>MGMEFSSHHIRLLQQLDEQRQKDLFCDCHIIVEGQMFKAHRNVLFASSGYFKMLLSQSCRDMGEPITATFDVFSADTFTAILDFVYSGKLPLSGQNVIEVMSAASYLQMTDVIGVCKMFIKSSLDINEKDRDGFFSLSDKDAGSNGSGLEHHHHHH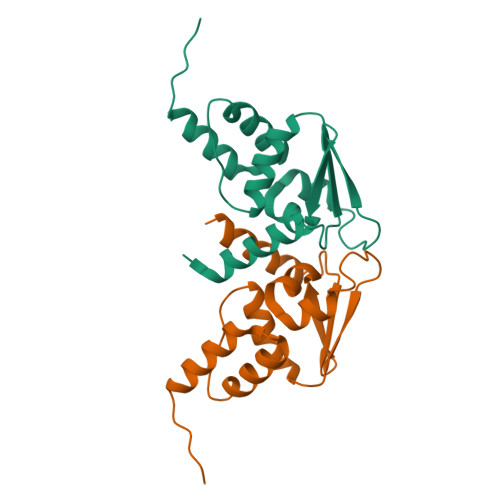[2x]> DVSGTVCLSALPPEATDTLNLIASDGPFPYSQDGVVFQNRESVLPTQSYGYYHEYTVITPGARTRGTRRIITGEAT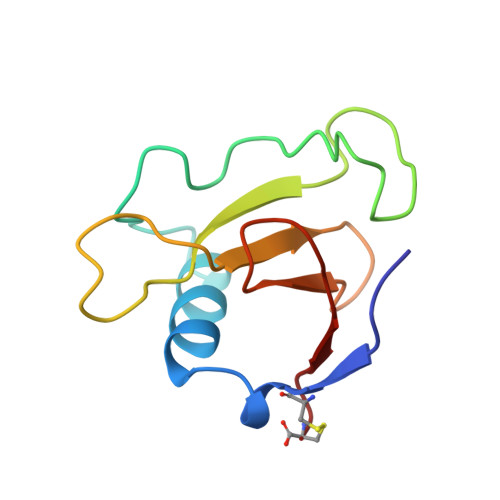QEDYYTGDHYATFSLIDQTC2-(1,3-DIOXO-1,3-DIHYDRO-2H-ISOINDOL-2-YL) ETHYL-4-(4'-ETHOXY 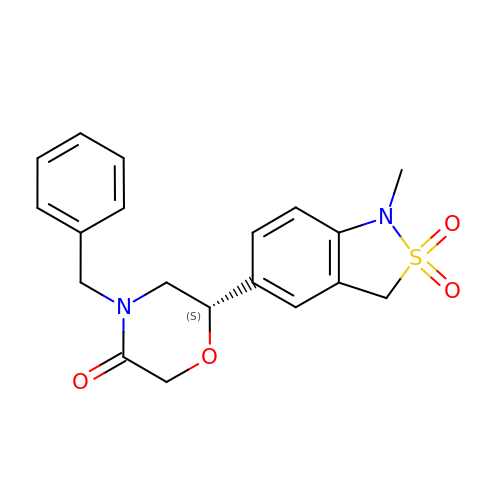[1,1'-BIPHENYL]-4-YL)-4-OXOBUTANOIC ACID | C19 H20 N2 O4 S | CIUMOGWIMXNXSQ-GOSISDBHSA-N> MSTSPGLAFANLTLLLDV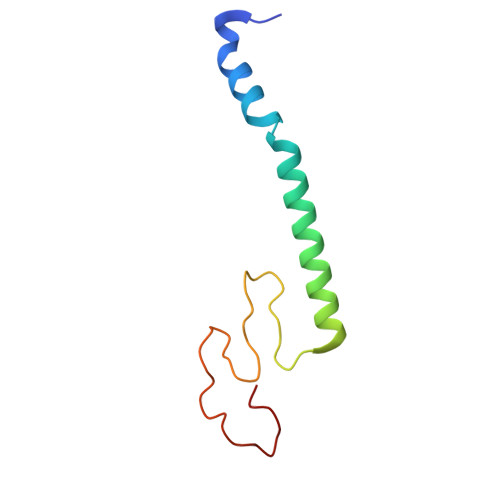PQLPAIWAVNAWRELNGLFTEMKTLAGTSDLLYPSNRYNPQNEKTNRMGRPRKYNHGEWMFGNSY>[2x]AASEDEFLRYLWRDYLYPKQYAWVLIAAYVAVFVVALVGNTLVCLAVWRNHHMRTVTNYFLVNLSLADVLATAICLPASLLVDITESWLFGHALCKVIPYLQTVSVSVAVLTLS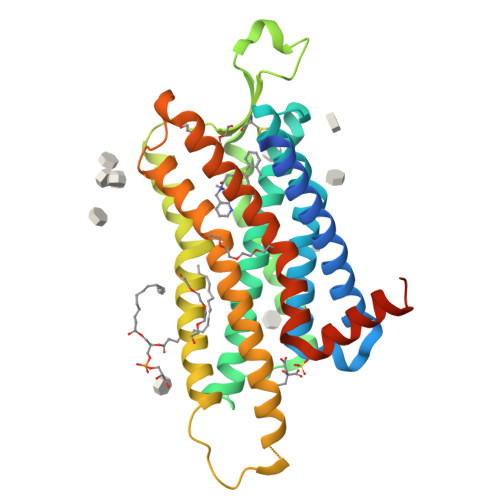FIALDRWYAICHPLLFKSTARRALGSILGIWAVSLAIMVPQAAVMECSSVLPELAARTRAFSVCDERWADDLAPKIYHSCFFIVTYLAPLGLMAMAYFQIFRKLWGRQIPGTTSAEVKQMRARRKTAKMLMVVVLVFALCYLPISVLNVLKRVFGMFRQASDREAVYAAFTFSHWLVYANSAANPIIYNFLSGKFREQFKAAFSWWLPGLAAAHHHHHHHHH>[2x]SMRAPQPVVARCKLVLVGDVQCGKTAMLQVLAKDCYPETYVPTVFENYTACLETEEQRVELSLWDTSGSPYYDNVRPLCYSD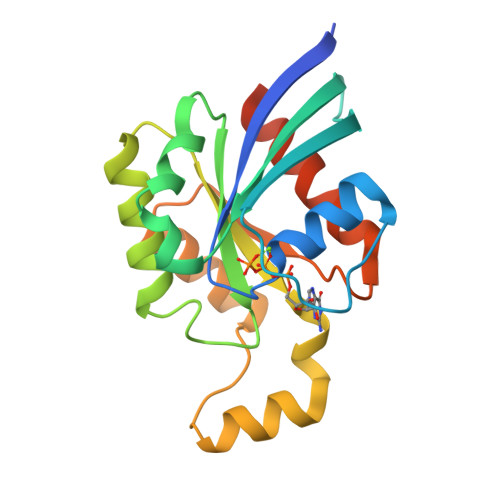SDAVLLCFDISRPETVDSALKKWRTEILDYCPSTRVLLIGCKTDLRTDLSTLMELSHQKQAPISYEQGCAIAKQLGAEIYLEGSAFTSEKSIHSIFRTASMLCLNKPSPLPQKSPV>[2x]MADKLFINALKKKFEESPEEKKTTFYTLGGWKQSERKTEFVNAGKEVAAKRGIPQYNPDIGTPLGQRVLMPYQVSTTDTYVEGDDLHFVNNAAMQQMWDDIRRTVIVGLNHAHAVIEKRLGKEVTPETITHYLETVNHAMPGAAVVQEHMVETHPALVADSYVKVFTGNDEIADEIDPAFVIDINKQFPEDQAETLKAEVGDGIWQVVRIPTIVSRTCDGATTSRWSAMQIGMSMISAYKQAAGEAATGDFAYAAKHAEVIHMGTYLPVRRARGENEPGGVPFGYLADICQSSRVNYEDPVRVSLDVVATGAMLYDQIWLGSYMSGGVGFTQYATAAYTDNILDDFTYFGKEYVEDKYGLCEAPNNMDTVLDVATEVTFYGLEQYEEYPALLEDQFGGSQRAAVVAAAAGCSTAFATGNAQTGLSGWYLSMYLHKEQHSRLGFYGYDLQDQCGASNVFSIRGDEGLPLELRGPNYPNYAMNVGHQGEYAGISQAPHAARGDAFVFNPLVKIAFADDNLVFDFTNVRGEFAKGALREFEPAGERALITPAK;>MAKFEDKVDLYDDRGNLVEEQVPLEALSPLRNPAIKSIVQGIKRTVAVNLEGIENALKTAKVGGPACKIMGRELDLDIVGNAESIAAAAKEMIQVTEDDDTNVELLGGGKRALVQVPSARFDVAAEYSAAPLVTATAFVQAIINEFDVSMYDA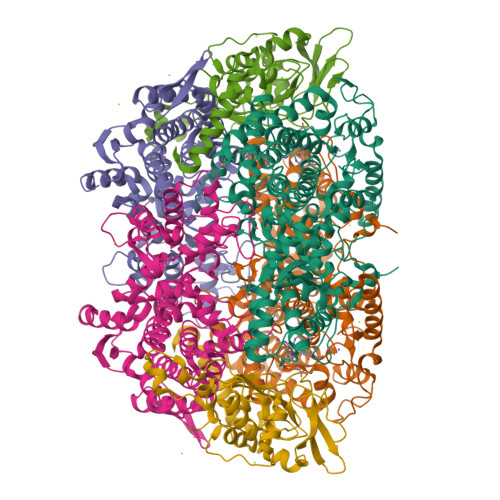NMVKAAVLGRYPQSVEYMGANIATMLDIPQKLEGPGYALRNIMVNHVVAATLKNTLQAAALSTILEQTAMFEMGDAVGAFERMHLLGLAYQGMNADNLVFDLVKANGKEGTVGSVIADLVERALEDGVIKVEKELTDYKVYGTDDLAMWNAYAAAGLMAATMVNQGAARAAQGVSSTLLYYNDLIEFETGLPSVDFGKVEGTAVGFSFFSHSIYGGGGPGIFNGNHIVTRHSKGFAIPCVAAAMALDAGTQMFSPEATSGLIKEVFSQVDEFREPLKYVVEAAAEIKNEI[2x];>MAQYYPGTTKVAQNRRNFCNPEYELEKLREISDEDVVKILGHRAPGEEYPSVHPPLEEMDEPEDAIREMVEPIDGAKAGDRVRYIQFTDSMYFAPAQPYVRSRAYLCRYRGADAGTLSGRQIIETRERDLEKISKELLETEFFDPARSGVRGKSVHGHSLRLDEDGMMFDMLRRQIYNKDTGRVEMVKNQIGDELDEPVDLGEPLDEETLMEKTTIYRVDGEAYRDDVEAVEIMQRIHVLRSQGGFNLE[2x]> AALEPTDSGAPSAIVMFPVSAKPNPKGAAMKPAVFNHLAHEKKIANCETCHHTGDPVACSTCHTTEGKAEGNF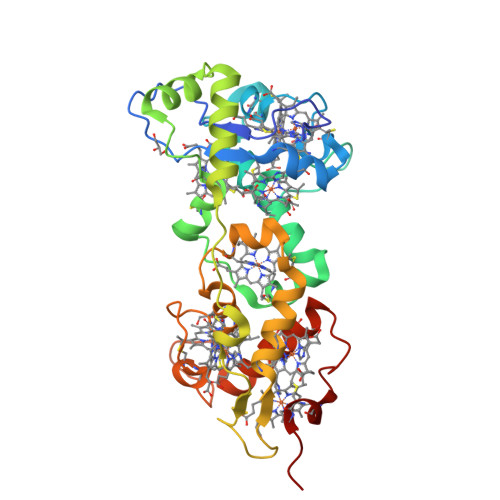VTLDRAMHATNIAKRAKGNTPVSCVSCHEQQTKERRECAGCHAIVTPKRDQAWCATCHNVTSSMTPEQMQQGIKGKLPPDQNEALAAETVLNHKPVQPLTAMQGPYKVSIDALADKYEPSNFTHRRHMASLMERIKGDKLAEAFHNKPETLCATCHHRSPLSATPPKCGSCHTKEIDPANPNRPNLKAAYHLQCMGCHQGMNVGRPKNTDCTTCHKARP Here, we identify and characterize a unique GlcN kinase from the soil bacterium Streptacidiphilus jiangxiensis, closely related to Streptomyces spp., the classical antibiotic producers. In contrast, from 20 sugars and 4 aminoglycoside antibiotics tested, SjGlcNK only phosphorylated specifically GlcN and displayed vestigial activity with glucose using ATP as a phosphate donor. Determination of the Michaelis constants (Km) for glucose and GlcN suggested that SjGlcNK is better described as a GlcN kinase (EC 2.7.1.8) with a strong preference for using GlcN (Km = 8 ± 1 mM) over glucose (Km > 100 mM) as the substrate. In addition, the structural and biochemical characterization of SjGlcNK provides new insights into the role of these unique GlcN kinases as the missing link for the incorporation of environmental GlcN to the metabolism of GlcNAc in bacteria, an important intermediate in peptidoglycan biosynthesis, glycolysis, and secondary metabolite production.

In crystals obtained by cocrystallization with a molar excess of ATP and GlcN, the substrates could be easily located in the electron density map, at the active site of the enzyme. Interestingly, this structure represents a snapshot of the phosphoryl transfer reaction in which ATP is hydrolyzed into ADP and inorganic phosphate (Pi), with the two hydrolysis products clearly identifiable in the electron density map. The ADP moiety is located in a cleft between the two lobes of SjGlcNK, which adopts a closed conformation, while both Pi and GlcN are found at the C-lobe. The adenine group binds to the hinge region, cross-linking the two lobes of the enzyme. In particular, the adenine establishes hydrophobic contacts with Y187 and L188 at the hinge, with V131, P164, and V185 at the intermediate subdomain, and with L307 and V316 at the C-lobe. The catalytic residues D317 (in the DFD loop) and Q305 (in the catalytic loop) coordinate the two magnesium ions, stabilizing this transition state. In this complex, the leaving phosphate is stabilized by D300 and the two magnesium ions, being perfectly oriented for transfer to position 6 of the bound sugar substrate, GlcN. Six conserved residues—W195, D300, H302, E409, Y412, and W420 (W222, D322, H324, E430, Y433, and W441 in MtMak)—mediate binding of the two sugars. In SjGlcNK, the amino group of GlcN is within hydrogen-bonding distance of the side chains of Q405 (K426 in MtMak) and E409 (E430 in MtMak).

>MTPNWSELVAAADPALVLPSGERRAEVAVPGPLRLDALLDLGEGHAVGVVRSADAARWTVPLVRDGAGGVRRSRPGDGTAEHLVAALARRGATPDAAFVLEAFTGAAPVTGERGIIVDQTNESVIVGECAVVKWAVRLPAEGEPGSPAAQRIAALARGGFTEMPRPWGLLTLAEGAQPVLLASVVAYLPGALDGWDWAVDDVRRLARGELTMDQALLPAAQLGTLTARMHAALAARGRTPATAADVAAWGVRMREELDEAVASVPGAEGERLKAWAPRIADVYAELDALAGTPLIDVHGDFHVGQILRADGRYAVVDFDGNPVLPADQRAARQPAALDVVGMTASLDHVGRVVVFRTPDVDPAPVRAWIAAAQRSFLDAYRTTLARLDADDLFDDRLLTPLRYAQEVREYLYAVRHLPHWVYVPDLSLTDLLPERLKDKLAAALEHHHHHH[2x]>MQYDHRSRDAFWQQKWDEKRIFDWDPSSPGKKFYVLEMFPYTSGHLHIGHVRNYSMGDTLARMQIARGYSVLHPMGWDSFGLPAENAARKFGTHPAKFTQDAIDSMKRSMMQLGFGYSWANELATCSPTYVLAQQKLFLDLYRKGLIYRDDTYVYWDPVEQTVLAAEQVIDGKGWRSGAAVYKRRTPQWFVDIRSYADRLLDDLESLEGWPTSVRNIQRNWIGRTEGAEVRFLVEASDLTINAFTTRLDTLAGCTFIALAPEHTILDELPIPSQMRASVKDYCESILVLSSEERSAGAKSGIFTGLMVVNPLNQERVPLYVANYVMPDFGTGAVIGVPAHDERDADFGALFGLPVRVVISTDSDATGLNIADGIVTNSHSLVDGLTSSAA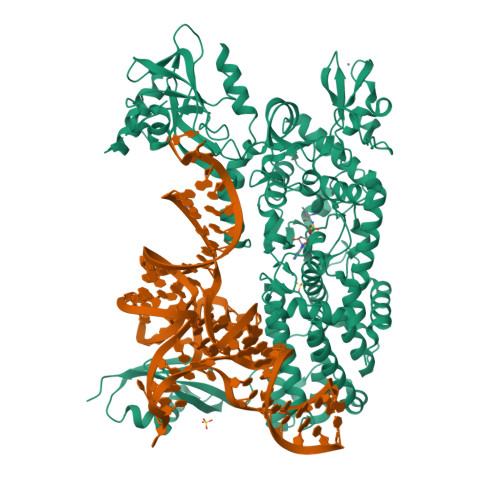REILIAHLSEKLEGQKSTQYRLQNWSISRQRYWGCPIPIIHCSECGTIPVAEEQLPILLPDHLISEGSGSPLSRDESWMKAKCPQCGGDAARDPDTMDTFVDSSWYFLRYPSPSSPNPIDSSLCNKIAPADVYIGGIEHATLHLIYSRFITKVLHDLGYIEFDEPFVELYNQGMVNDVHGRKQSKSLGNVTDPSVVVQEFGADAVRCYLLFKTTYNAPINWEDSGPQAMRSYLERVCRLFTNNLDRLRSSSAIEICPDDCENEEDREIARQLQLAIGKVTADVERFHFNAAIAAIMSVTNLLYEKGGKASPTVLAGSLRLLVRLLAPFAPHISEELWALSGCNSLVAAEPWPTINERLVQAENIVLPVQINGKLIRTMTIPVNLAEEDILSTVLALPEVRSRLSDRDLKNYRYVPNRIINLVVGLEHHHHHH[2x]> MPELPEVETIRRTLLPLIVGKTIEDVRIFWPNIIRHPRDSEAFAARMIGQTVRGLERRGKFLKFLLDRDALISHLRMEGRYAVASALEPLEP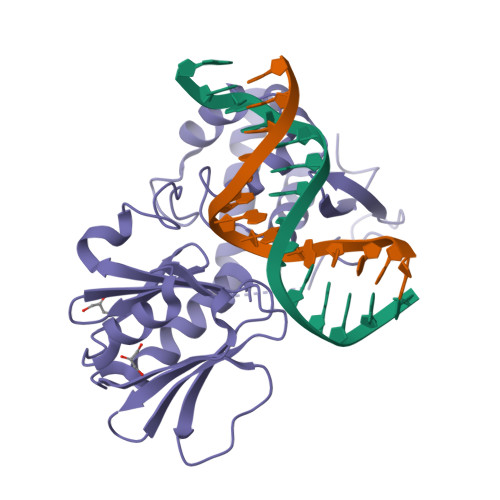HTHVVFCFTDGSELRYRDVRKFGTMHVYAKEEADRRPPLAELGPEPLSPAFSPAVLAERAVKTKRSVKALLLDCTVVAGFGNIYVDESLFRAGILPGRPAASLSSKEIERLHEEMVATIGEAVMKGGSTVRTYVNTQGEAGTFQHHLYVYGRQGNPCKRCGTPIEKTVVAGRGTHYCPRCQR>NANRSKEWKNAANTLLFGLDESVDPCEDFYGFTCNKFIERIDLDELGRGRFTTFSQAQLEVNSDIVKALEKVDVNDEKFSQTERITKAAFQSCVEYTLKDDRKASVNELLQYISERFGGIPFLGQRVKGGCELYREMGRIEQQRALPTFMYTWVNVDHKNVSRNSYYISQPTLPMPREFYVLPQFAPELDARTKAIENVMKAFASDILKDPSKYDKMIKTAAREVTQIEQKIAMASWPDDELRNHEQQYNPYELFAPSEGKIALQDAFPNIRFGKYIAGLMETATGGVPVSPVFIGDVIVTNPAYMGFLNTLFRQTNIQMNQYPFVNYIIVHMLFEDAEHLGDKYLRIAKDADYVTYAQRKGVGITRSGRKYSRVFDERTDARMKCVDTITTYMPYGTGYVYVNSREDRDQVVEDVKQQTELIMKTFLKKMLSTLSWMQGESYRRAEKKINEMHRNYGWPKKLFGDFKNFDTIDAYHRDDYYSILEAYNNKTDKSTAFYTILNILRRGYENRESFRRKNETADRTNFLESPASVNAWYAPELNSLTLPFGILTSPHYDLQFPKAFNFAGSGTVGGHELVHGFDDEGVQFDYDGSLADCSVYECGWLEQKGKNGFKDMAQCVVTQYNAQCCPAKEGNVHCANGAHTQGENIADLGGLQASYNAYKEYIKMKGAEEMRLPGLEKFTPNQIFWISYGYSWCAKETQSSLVKRLLTNPHSPNSCRVNQVLQDIPSFAKDFQCALGQKMYPPAEQRCKVW[4x];>VFPHPIYDYQDTEYLAKITIGAPGQSFHVVLDTGSANLWIPDNICVNGRRGACRITTCDRGLVCEVLCHDKSCCEDDVDNPDEDNPCKGKSGFDSTQSTSYAKITPKKYFEIVYGTGFAKGFLGNDTVRFGEEGNNKTLVVPGTVFGQAVQIGDPFANNPINGILGLGFRGLAQAGVTPPLQRAIDLKLVDPIFTVYMKQLGAKAKGQDGGAFTYGGLDSVNCGQEIAYVDLTRPLYWQFKMEAFSAGYLSIRKGWEVISDTGTSFMGVPTAIADLVADSYGGQYDEMFEIYTVDCNATVTFGMTIGGKQYKIERKNLVLEEDKDSCMIAMTPLSSVGFGPQWILGAPFIRQYCNIHDMRNNTIGFAEP[2x];> DPDIPENYDPRLIWPNCSSLFTIPDQANCGSCWAVSTAAAISDRLCIASKGENQVFISSADILSCCDTCGFGCDGGITFRAWEYFATKGSVSGGHFEAPNCCRPYYFHPCGQHGNDTFYGYCPRFAQTPFCRRKCRIGFNKSYAQDRIQGKSFYTVDYSVPAIQREIMTKGSVVGSYDVFTDFSHYKSGIYRHTGGKPDGRHAVRIIGWGKENGTDYWLIANSWHDDWGENGYFRMIRGINDCGIEQDITAGD

A major Barbervax component is H-gal-GP (Haemonchus galactose containing glycoprotein complex), which is highly protective in sheep vaccine trials. H-gal-GP is located in the luminal brush border of the nematode gut and digests ovine hemoglobin and albumin, major components of the Haemonchus blood meal. A combination of SDS-PAGE, N-terminal sequencing and cDNA library screening, have shown that H-gal-GP is composed primarily of families of two aspartyl proteases (PEPs 1 or 2), four metalloproteases (MEPs 1, 2, 3 or 4) and several cysteine proteinases (CPs). H-gal-GP is a multi-enzyme protease complex that digests the Haemonchus blood meal.

The final reconstruction of H-gal-GP at 4.5 Å global resolution was extracted from approximately 60% of the particles by classification with masking of the core base region. The reconstruction revealed that H-gal-GP has, to the best of our knowledge, a novel architecture, a central base with two ‘wings’ and an archway, giving rise to a cavity in the middle of the complex. The base has a series of channels connecting to the central cavity. Once docked, models were refined with molecular dynamics flexible fitting (MDFF). Both aspartyl proteases (PEP1 and PEP2) fit well within the arch, which is not sufficiently bulky to accommodate any of the metalloproteases. The PEP1 model was docked into the map as the model for PEP2 was almost identical. Since the MEP models were all similar in tertiary structure, four copies of MEP3 were docked into the central base. A single CP was accommodated with reasonable agreement into the wing. The proposed active sites of PEP1 protrude into the central cavity of the complex whose dimensions are large enough to accommodate hemoglobin (Hb) or albumin. The channels through the centre of the base would allow for fragments of Hb to enter the active sites of the MEPs and exit through the bottom of the base. The architecture accommodates a sequential digestion pathway, facilitating positioning of products from initial digestion for subsequent digestion by the next enzyme in the pathway.> MSLATQQLGIIGLFVPTFFGSYYGTILKQTDLELRAVHRHVVVATGCGESTPREQALEAVRFLIGRDCDGVVVISHDLHDEDLDELHRMHPKMVFLNRAFD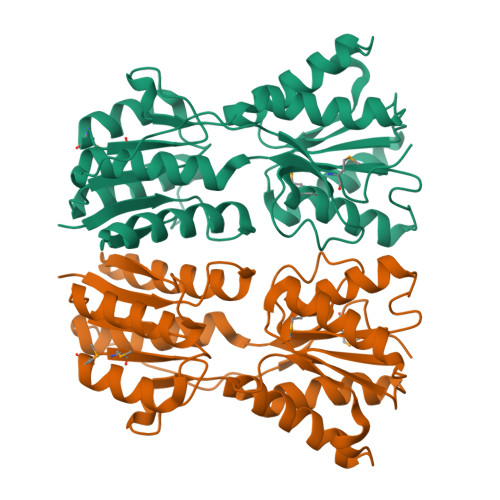ALPDASFCPDHRRGGELAAATLIEHGHRKLAVISGPFTASDNVERLDGFFDELARHGIARDSVPLIESDFSPEGGYAATCQLLESKAPFTGLFCANDTMAVSALARFQQLGISVPGDVSVIGYDDDYSAAYAAPALTSVHIPTAELTQNAVRWLINQCYGTKWEIFREFPVTVSMRASVAREGHHHHHH>[2x]MDEKRRAQHNEVERRRRDKINNWIVQLSKIIPDSSMEST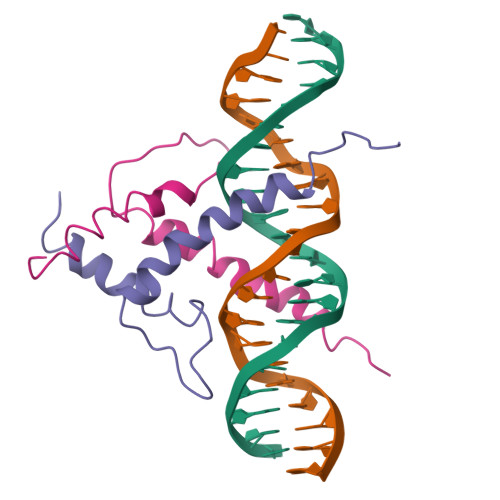KSGQSKGGILSKASDYIQELRQSNHR> MVSVIDKLVFDFGGKTLVSLAPDNNTLCVANKNGLTKILKTNNPEEEPETLDSSKLVSSIKCYSNSHFLMTTMQGDALRYNIDSSQEELLARFALPLRDCCVIHSGKMAVFGGDDLELILLELDDETHKKHAIKIDEQVSQISYNSQMNILAVSMINGKVQIFSLTSTIPNKVHELNDYIVANSYDDTHRDKILSNMMDDIDKDNDNDLSETADPDENNVADPEFCAANRICTRVAWHPKGLHFALPCADDTVKIFSIKGYSLQKTLSTNLSSTKAHFIDLQFDPLRGTYIAAVDLNNKLTVWNWETSEIHYTREFKRKITNIAWKIQADSKTLDLVLGTWSGSIAIVQNLAESVVSNIPDQSVAESSTKHGLFVDSESDLENLEGNDDINKSDKLFSDITQEANAEDVFTQTHDGPSGLSEKRKYNFEDEE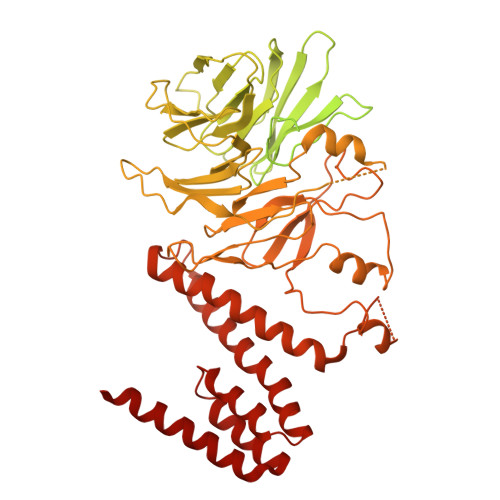DFIDDDDGAGYISGKKPHNEHSYSRVHKTHSFPISLANTGKFRYMPFSPAGTPFGFTDRRYLTMNEVGYVSTVKNSEQYSITVSFFDVGRFREYHFEDLFGYDLCFLNEKGTLFGQSKTGQIQYRPHDSIHSNWTKIIPLQAGERITSVAATPVRVIVGTSLGYFRSFNQFGVPFAVEKTSPIVALTAQNYRVFSVHYSQFHGLSYSLSELGTSSKRYYKRECPLPMSLPNINSDMKKDANLDYYNFNPMGIKSLFFSSYGDPCIFGSDNTLLLLSKWRSPEESKWLPILDSNMEIWKMSGGKETTDIHVWPLALAYDTLNCILVKGKHIWPEFPLPLPSEMEIRMPVFVKSKLLEENKAILNKKNEIGADTEAEEGEEDKEIQIPVSMAAEEEYLRSKVLSELLTDTLENDGEMYGNENEVLAALNGAYDKALLRLFASACSDQNVEKALSLAHELKQDRALTAAVKISERAELPSLVKKINNIREARYEQQLK> LRPVLPTQSAHDPPAVHLSNGPGQEPIAVMTFDLTKITKTSSSFEVRTWDPEGVIFYGDTNPKDDWFMLGLRDGRPEIQLHNHWAQLTVGAGPRLDD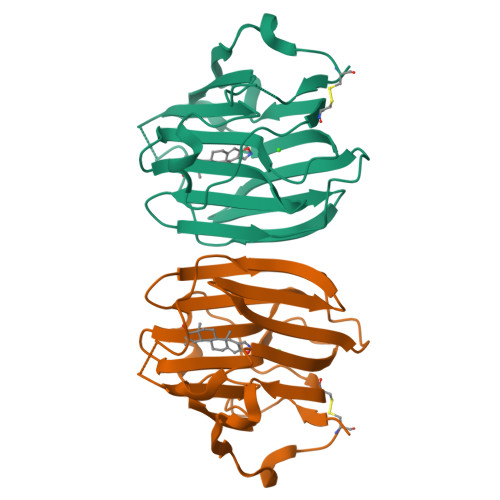GRWHQVEVKMEGDSVLLEVDGEEVLRLRQVSGPLTSKRHPIMRIALGGLLFPASNLRLPLVPALDGCLRRDSWLDKQAKISASAPTSLRSCDVESNPGIFLPPGTQAE(2S)-1-(4-azanylpiperidin-1-yl)carbonyl-N-(2-cyclopropylethyl)-2-methyl-4-oxidanylidene-3,5-dihydro-2H-1,5-benzodiazepine-7-carboxamide | C22 H31 N5 O3 | 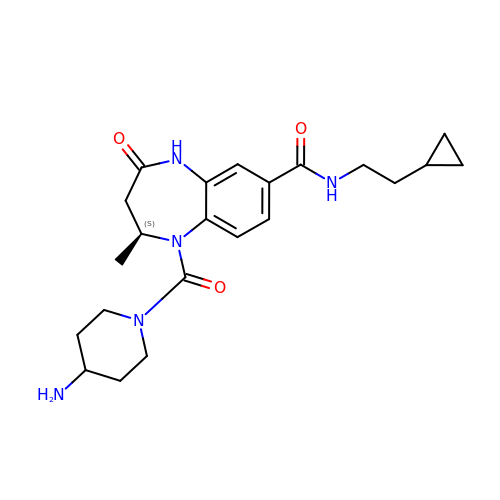YEYZZZLQSMITHG-AWEZNQCLSA-N> CACGAGCCTGATCGGACAAGATCCGCTAGCG;> G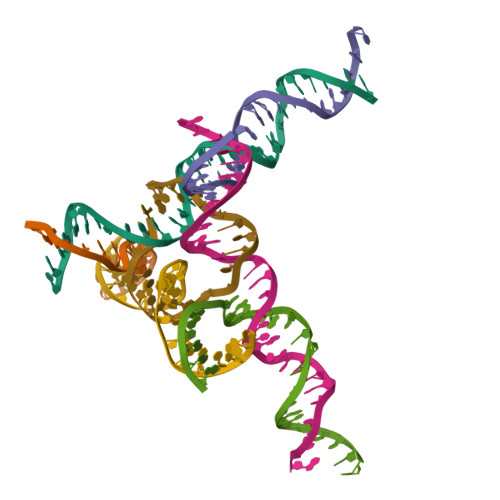AGCAGCCTGTACGGACATCAGTCTATGCTA;> AACCTACCTGGCAGGACGACT;> TGCGCTAGCGGATCTTGTGGCTGC;> TTAGTCGTGGCTCG;> TCTAGCATAGACTGATGTGGTAGG;> TCACCTGCCACCGTACACCGA> KRQVASGRAYIHASYNNTIVTITDPDGNPITWSSGGVIGYKGSRKGTPYAAQLAALDAAKKAMAYGMQSVDVIVRGTGAGREQAIRALQASGLQ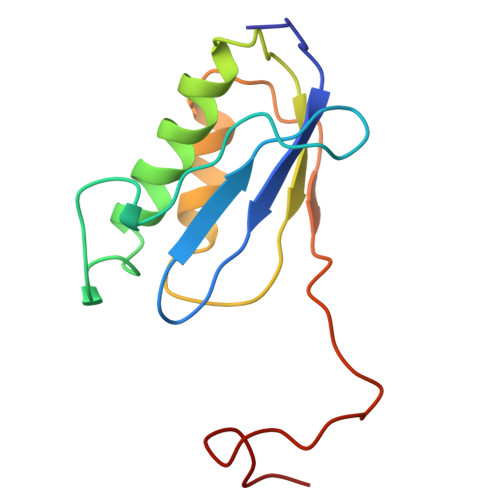VKSIVDDTPVPHNGCRPKKKFRKAS> MSMSKQVLKEDMKMTYHMDGSVNGHYFTIEGEGTGNPFKGQQTLKLRVTKGGPLPFAFDILSPTFTYGNRVFTDYPEDMPDYFKQSLPEGYSWERTMMYDDGASATASARISLDKNGFVHKSTFHGENFPANGPVMKKKGVNWEPSSETITASD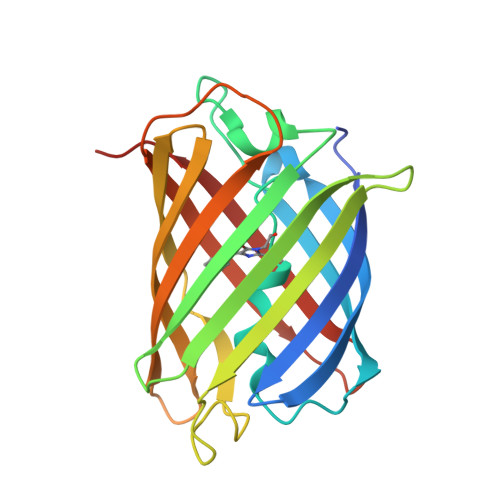GILKGDVTMFLVLEGGQRLKALFQTTYKANKVVKMPPRHKIEHRLVRSEDGDTVQLQEHAVAKYFTV>[2x]GAMNAQAEEFKKYLETNGIKPKQFHKKELIFNQWDPQEYCIFLYDGITKLTSISENGTIMNLQYYKGAFVIMSGFIDTETSVGYYNLEVISEQATA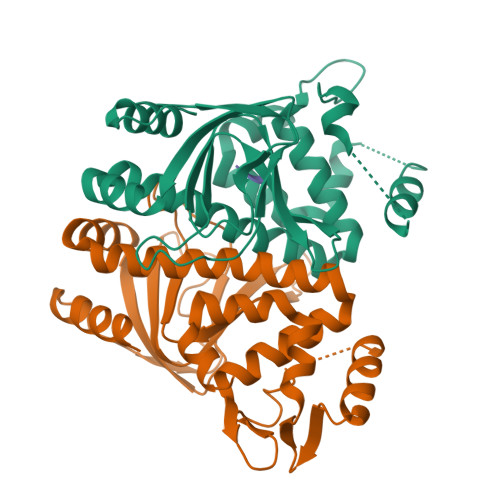YVIKINELKELLSKNLTHFFYVFQTLQKQVSYSLAKFNDFSINGKLGSICGQLLILTYVYGKETPDGIKITLDNLTMQELGYSSGIAHSSAVSRIISKLKQEKVIVYKNSCFYVQNLDYLKRYAPKLDEWFYLACPATWGKLN;> TEPL Rspo (R-spondin, also roof plate-specific spondin) proteins are evolutionarily conserved from fish to humans and have well-documented roles in a broad range of developmental and physiological processes resulting from enhancement of canonical and non-canonical Wnt signalling. ZNRF3/RNF43 specifically targets these Wnt receptors for ubiquitination and turnover, hence reducing Wnt signalling responses. Direct extracellular interaction with Rspo proteins inhibits ZNRF3/RNF43 activity. Here we report a molecular level analysis of the ZNRF3/RNF43 ectodomain structure and its interactions with Rspo proteins.

The ZNRF3ecto crystal structures revealed a distinctive variant of the protease-associated domain topology. Two β-sheets (comprising β2, β1, β7, β3 and β4, β5, β6 strands, respectively) splay apart, accommodating an α-helix (αC) at the open edge; two additional α-helices (αA and αB) pack against the β4, β5 and β6 face of this distorted β-sandwich. A disulphide bridge, conserved across species, links two structurally elaborate loops, β3–β4 and β4–αA. The crystal structures for apo xZNRF3ecto, zZNRF3ecto and mZNRF3ecto showed no major differences in the main chain conformation. Comparisons of ZNRF3ecto structures for proteins crystallized in several different crystal lattices, or for crystals containing multiple copies in the asymmetric unit, consistently highlighted an acidic region (N105-E114; residue numbering is for mouse sequences unless otherwise stated) within the β3–β4 loop, the short αC–β7 loop and the extended β1–β2 hairpin as flexible elements of the fold. Our crystallographic data provided independent structures for multiple copies of the ZNRF3 ectodomain in eight different crystal forms. All but two of these crystal structures reveal an extensive interface (average interface area 992±109 Å2) formed between two ZNRF3ecto polypeptide chains. This dimer is conserved, and pairwise structural superpositions yielded r.m.s.d. values of <1.3 Å (for 275 equivalent Cα pairs). The interaction is twofold symmetric; strands β3 and β7 of the ‘subunits’ abut face-to-face at the core of the dimer. The β1–β2 hairpin forms a second interface by reaching out to embrace helix αA and the β3–β4 loop in the opposing subunit.

>[4x]ETGKETAFVEVVLFESSPSGDYTTHTTGLTGRFSRAGAMLSAEGEIVQMHPLGLCNNNDEEDLYEYGWVGVVKLEQPELDPKPCLTVLGKAKRAVQRGATAVIFDVSENPEAIDQLNQGSEDPLKRPVVYVKGADAIKLMNIVNKQKVARARIQHLGTKHHHHHH Mtb Decaprenylphosphoryl‐β‐d‐ribofuranose 2‐oxidase (DprE1) is a flavin adenine dinucleotide (FAD)‐dependent enzyme, which together with decaprenylphosphoryl‐d‐2‐ketoerythropentose reductase (DprE2), converts decaprenylphosphoryl‐beta‐d‐ribose (DPR) to decaprenylphosphoryl‐beta‐d‐arabinofuranose (DPA), an essential cell wall component. Multiple covalent3 and non‐covalent4 DprE1 inhibitors have been identified and showed in vitro and in vivo activities against Mtb, further validating DprE1 as an attractive anti‐tuberculosis (TB) drug target. When analyzing toxicity profiles, we noticed that many TCA1 analogs show inhibition of CYP2C9, one of six major cytochrome P450 enzymes which determine the clearance of 75 % of marketed drugs. Here we report the X‐ray crystal structures of WT DprE1, a TCA1‐resistant DprE1 mutant, and CYP2C9 in complex with TCA1 analogs.

Y314 resides close to the carbamate moiety and it was previously found that a spontaneous TCA1 resistant mutant harbors a Y314C mutation. We measured the inhibitory activities of TCA1 and its analogs against DprE1 and the Y314C variant and observed 5‐ to 40‐fold shift on IC50 values under the same assay condition, which is consistent with the MIC shift between the wildtype (WT) and the mutant strain. We also generated a Y314A mutant and it is sensitive to TCA1 inhibition, suggesting that the side chain of Y314 does not directly contribute to TCA1 binding. To elucidate the molecular basis of the resistance mechanism, the structure of DprE1 Y314C bound with TCA1 was determined to 2.2 Å. Although the overall fold of the mutant enzyme is identical to wildtype, consequential structural changes in the active site of DprE1 were evident. The most striking difference between the WT and mutant DprE1 complexes is the 180° flipped orientation of the boomerang‐shaped ligand in the active site. The alternative orientation of the ligand can be linked to the effects of cysteine 314 substitution on the orientation of Lys134, which positions the ϵ‐ammonium group in the void created by substituting the tyrosyl ring with a thiol. The reorientation of Lys134 is driven by formation of a strong H‐bond (2.75 Å) between its ϵ‐ammonium and the thiol of Cys314 and results in a noticeable shape change of the active site around Lys134. Consequently, the acylcarbamate keto‐oxygen in the original orientation would clash with the alkyl moiety of Lys134 (with the shortest distance at 2.7 Å), which likely weakens the binding of TCA1.

>MGSSHHHHHHSQDPNSMLSVGATTTATRLTGWGRTAPSVANVLRTPDAEMIVKAVARVAESGGGRGAIARGLGRSYGDNAQNGGGLVIDMTPLNTIHSIDADTKLVDIDAGVNLDQLMKAALPFGLWVPVLPGTRQVTVGGAIACDIHGKNHHSAGSFGNHVRSMDLLTADGEIRHLTPTGEDAELFWATVGGNGLTGIIMRATIEMTPTSTAYFIADGDVTASLDETIALHSDGSEARYTYSSAWFDAISAPPKLGRAAVSRGRLATVEQLPAKLRSEPLKFDAPQLLTLPDVFPNGLANKYTFGPIGELWYRKSGTYRGKVQNLTQFCHPLDMFGEWNRAYGPAGFLQYQFVIPTEAVDEFKKIIGVIQASGHYSFLNVFKLFGPRNQAPLSFPIPGWNICVDFPIKDGLGKFVSELDRRVLEFGGRLYTAKDSRTTAETFHAMYPRVDEWISVRRKVDPLRVFASDMARRLELL[2x]[5,5-dimethyl-3-(2-methylphenyl)-4~{H}-pyrazol-1-yl]-pyridin-4-yl-methanone 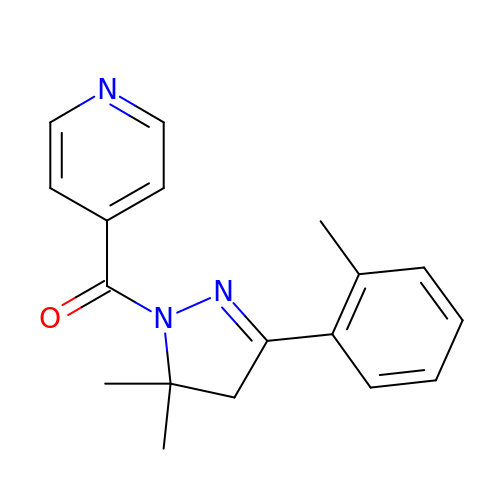| C18 H19 N3 O | YQBXKJJOBGJGKY-UHFFFAOYSA-N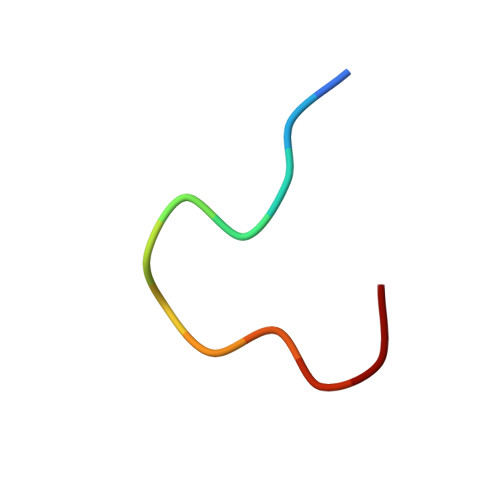> DVFYPYPYASGS{(2R)-2-{2-[hydroxy(methyl)amino]-2-oxoethyl}-5-[4-(trifluoromethyl)phenyl]pentyl}phosphonic acid | C15 H21 F3 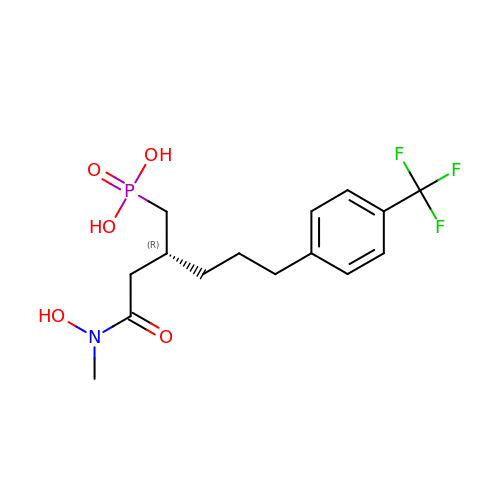N O5 P | QJHOMBPUEUGKSC-GFCCVEGCSA-N>[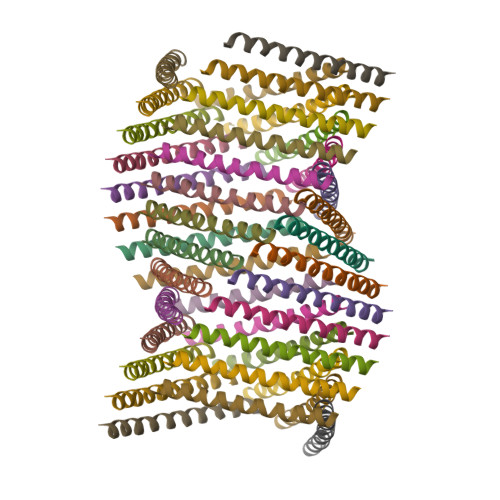41x]TLEELRAEARILEAKAEILKAKAEVLKAKAEILKAQ> MDAQAAARLGDEIAHGFGVAAMVAGAVAGALIGAAV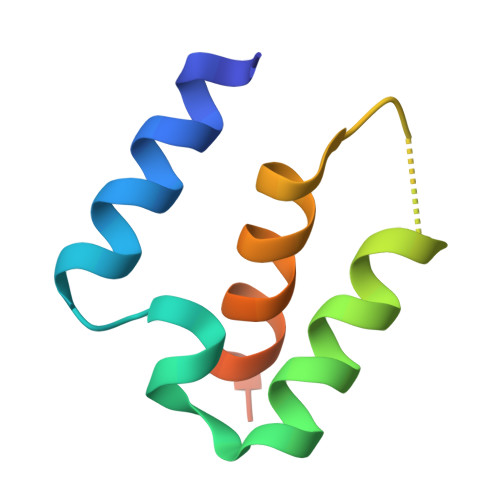VAATAATGGLAAVILAGSIAAGGLSHHHHHH> SSNTPRFK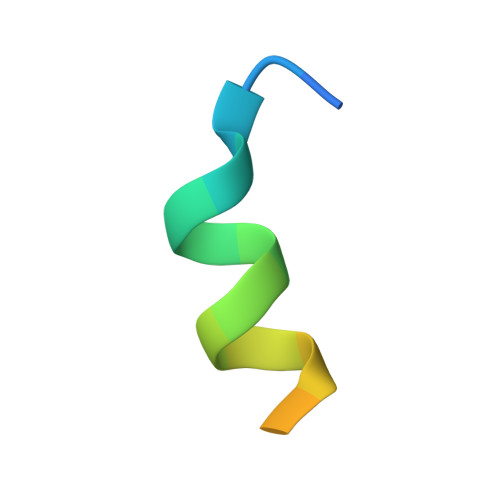EYFMQSRSGSGK>[2x]MAEIPKEMLRAQTNVILLNVLKQGDNYVYGIIKQVKEASNGEMELNEATLYTIFKRLEKDGIISSYWGDESQGGRRKYYRLTEIGHENMRLAFESWSRVDKIIENLEANKKSEAIKHHHHHH

LmrR is a transcriptional repressor regulating the expression of the multidrug ABC transporter LmrCD. In the apo state, LmrR shows high affinity for the promotor region of LmrRCD. This affinity is reduced upon binding of a drug at its drug-binding site, enabling expression of the multidrug transporter. LmrR is a homodimeric protein with the drug binding site at the dimer interface.19 Central in this binding site are two Trp residues, W96 and W96′ (residue 96 from the other monomer), oriented face-to-face at 7 Å from each other.

The LmrR protein contains two unique Trp residues, W96 in the drug binding site and W67 at a solvent exposed position, approximately 30 Å away from W96 and the drug binding site. Thus, W67 is not involved in drug binding. To investigate the importance of π–π interactions for drug binding, the electron density in the π electron cloud of W96 was modulated by progressive fluorination of the W96 indole side chain. By our method, all Trp residues that are present in a protein are replaced by a Trp analog, thus making the system most suitable for proteins containing a limited number of Trp residues. We obtained milligram quantities of pure, labeled protein, which allowed, for the first time, the crystallization and structure determination of a set of proteins labeled with mono-, di-, or trifluoroTrp. It provided detailed insights into the effects of fluorination on the binding interactions of the indole side chain.> MKVVTGKSIKEVDKNELVNILNAYKKVEVDLGTGDGRYVYKNAKENSGTLFIGIEPIQKQLENYSRKSQKENITNAIYILGSVEYFPDELLGTADKLTIILPWGSLLQSITNPNYEKNSLISNILKSNGICEIVLGYSQEYEPNETERLELENLSVEYLKSTVIPIFEKNNLHLTEFGSLGK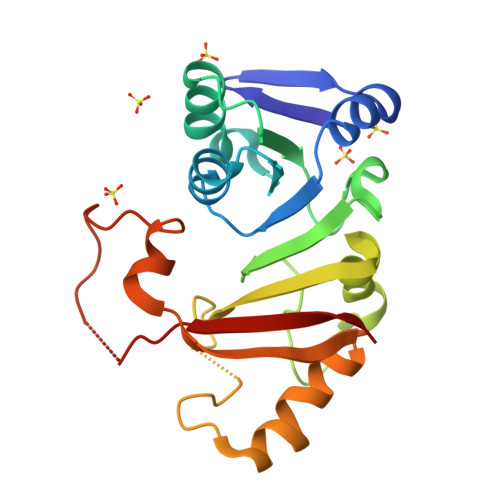KDLKPIESTWSKKLSFGKNRPLYQLKFKKMLN>[2x]HMDEILARAGIFQGVEPSAIAALTKQLQPVDFPRGHTVFAEGEPGDRLYIIISGKVKIGRRAPDG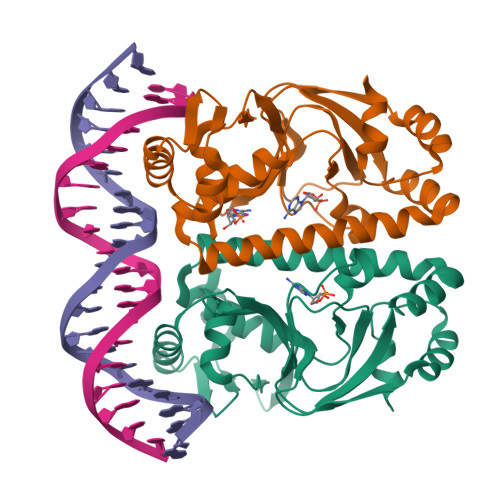RENLLTIMGPSDMFGELSIFDPGPRTSSATTITEVRAVSMDRDALRSWIADRPEISEQLLRVLARRLRRTNNNLADLIFTDVPGRVAKQLLQLAQRFGTQEGGALRVTHDLTQEEIAQLVGASRETVNKALADFAHRGWIRLEGKSVLISDSERLARRAR> MKTKPLPTAPMAWAESAVETTTSPRELAGHAPLRRVLRPPIARRDGPVLLGDRAPRRTASTMWLLGIDPAESSPGTRATRDDTEQAVDKILRGARRAGGLTVPGAPRYHLTRQVTLTDLCQPNAERAGALLLALRHPTDLPHLARHRAPPGRQTERLAEAWGQLLEASALGSGRAESGCARAGLVSFNFLVAACAAAYDARDAAEAVRAHITTNYGGTRAGARLDRFSECLRAMVHTHVFPHEVMRFFGGLVSWVTQDELASVTAVCSGPQEATHTGHPGRPRSAVTIPACAFVDLDAELCLGGPGAAFLYLVFTYRQCRDQELCCVYVVKSQLPPRGLEAALERLFGRLRITNTIHGAEDMTPPPPNRNVDFPLAVLAASSQSPRCSASQVTNPQFVDRLYRWQPDLRGRPTARTCTYAAFAELGVMPDDSPR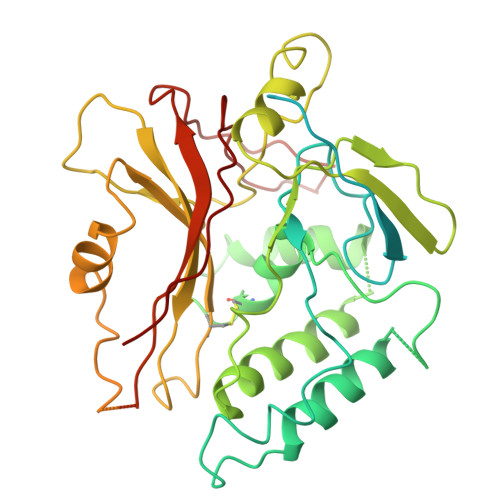CLHRTERFGAVGVPVVILEGVVWRPGGWRACA> KN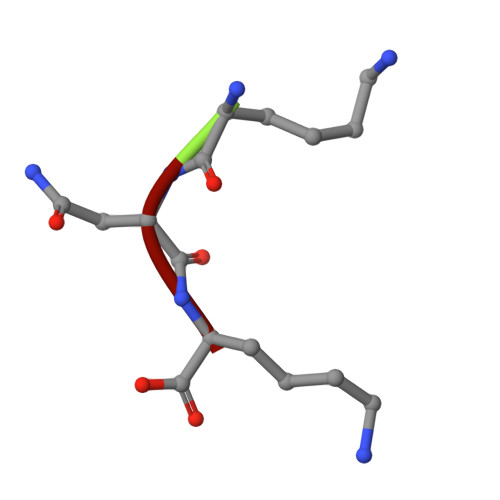K>[2x]MVGKVKVENI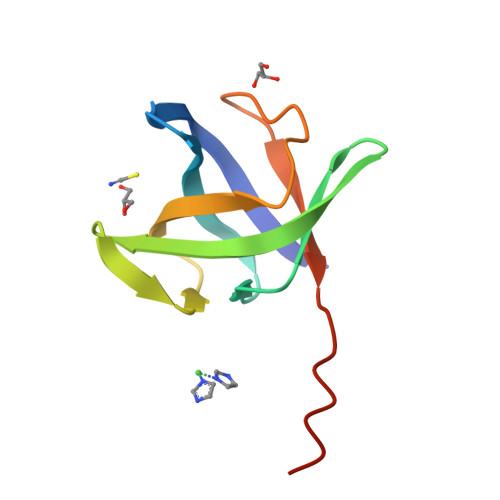LIVGFKTVIICEVLEGMVKVGYKVRKGKKVAGIVSMEREHKKVEFAIPGDKIGIMLEKNIGAEKGDILEVFIVLEHHHHHHH>[3x]SGPAATNKRHSTSDKMHFPRSSLQPITTLGKSEFGEVFLAKAQGLEEGVAETLVLVKSLQSKDEQQQLDFRRELEMFGKLNHANVVRLLGLCREAEPHYMVLEYVDLGDLKQFLRISKSKDEKLKSQPLSTKQKVALCTQVALGMEHLSNNRFVHKDLAARNCLVSAQRQVKVSAL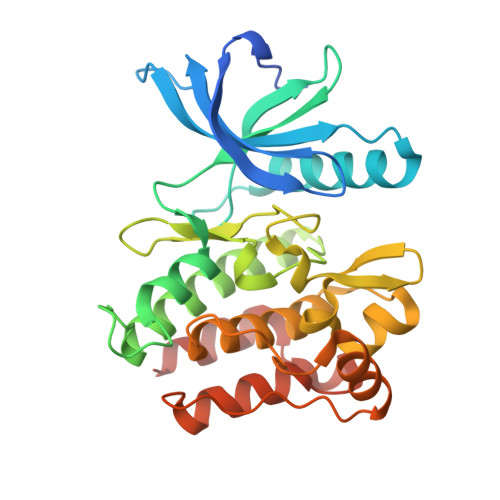GLSKDVYNSEYYHFRQAWVPLRWMSPEAILEGDFSTKSDVWAFGVLMWEVFTHGEMPHGGQADDEVLADLQAGKARLPQPEGCPSKLYRLMQRCWALSPKDRPSFSEIASALGDSTVDSK> ERFDAFI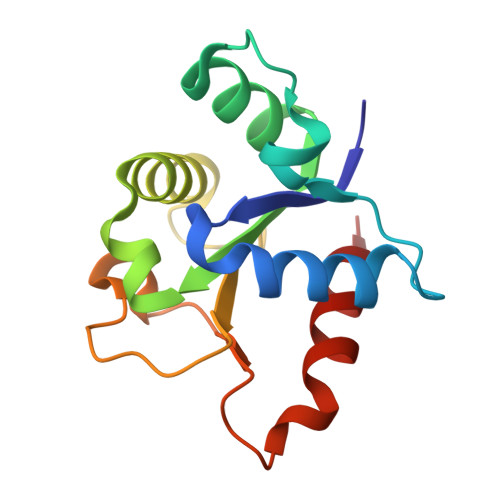CYCPSDIQFVQEMIRQLEQTNYRLKLCVSDRDVLPGTCVWSIASELIEKRCRRMVVVVSDDYLQSKECDFQTKFALSLSPGAHQKRLIPIKYKAMKKEFPSILRFITVCDYTNPCTKSWFWTRLAKALSLP> MSKLASPQSVRALLERHGLFADKRFGQNFLVSEAHLRRIVEAARPFTGPVFEVGPGLGALTRALLEAGAEVTAIEKDLRLRPVLEETLSGLPVRLVFQDALLYPWEEVPQGSLLVANLPYHIATPLVTRLLKTGRFARLVFLVQKEVAERMTARPKTPAYGVLTLRVAHHAVAERLFDLPPGAFFPPPKVWSSLVRLTPTGALDDPGL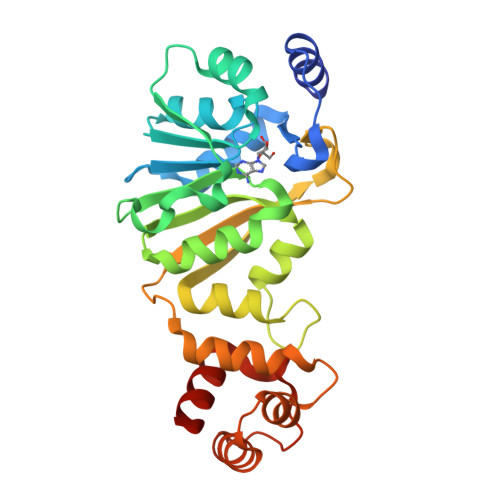FRLVEAAFGKRRKTLLNALAAAGYPKARVEEALRALGLPPRVRAEELDLEAFRRLREGLEGAV> MAPTWFYNTTNSEKLRELQHVLGGSAKLGYLTAKVTEILDVDLETV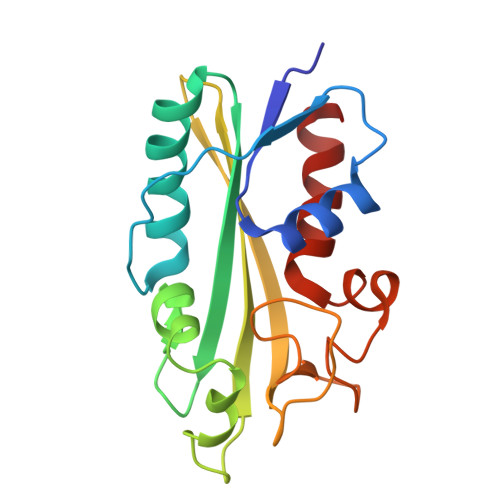IRAKAIAAYRAVRVPVIVEHGALCIDALNGLPGALVKPFWESLDTRLCEVIPAGQRTARARGALCYCDGRERHVLIEETEGEIAPSARGTGGFHWDPIFIPKGQTRTFAEMSLDEKLSFSPLGRLHTRLRTELGL>AEYCKMKKDYRKKYRKYVRSRFQCIEDRNARLGESVSLNKRYTRLRLIKEHRSQQEREQELLAIGKTKTCESPVSPIKMELLFDPDDEHSEPVHTVVFQGAAGIGKTILARKMMLDWASGTLYQDRFDYLFYIHCREVSLVTQRSLGDLIMSCCPDPNPPIHKIVRKPSRILFLMDGFDELQGAFDEHIGPLCTDWQKAERGDILLSSLIRKKLLPEASLLITTRPVALEKLQHLLDHPRHVEILGFSEAKRKEYFFKYFSDEAQARAAFSLIQENEVLFTMCFIPLVCWIVCTGLKQQMESGKSLAQTSKTTTAVYVFFLSSLLQPRGGSQEHGLCAHLWGLCSLAADGIWNQKILFEESDLRNHGLQKADVSAFLRMNLFQKEVDCEKFYSFIHMTFQEFFAAMYYLLEEEKEGRTNVPGSRLKLPSRDVTVLLENYGKFEKGYLIFVVRFLFGLVNQERTSYLEKKLSCKISQQIRLELLKWIEVKAKAKKLQIQPSQLELFYCLYEMQEEDFVQRAMDYFPKIEINLSTRMDHMVSSFCIENCHRVESLSLGFLHNMPKEEEEEEKEGRHLDMVQCVLPSSSHAACSHGLVNSHLTSSFCRGLFSVLSTSQSLTELDLSDNSLGDPGMRVLCETLQHPGCNIRRLWLGRCGLSHECCFDISLVLSSNQKLVELDLSDNALGDFGIRLLCVGLKHLLCNLKKLWLVSCCLTSACCQDLASVLSTSHSLTRLYVGENALGDSGVAILCEKAKNPQCN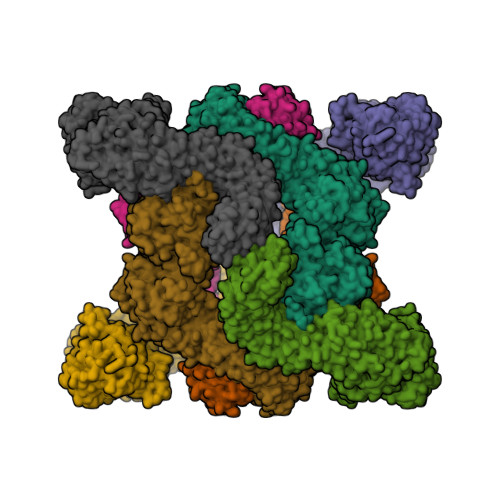LQKLGLVNSGLTSVCCSALSSVLSTNQNLTHLYLRGNTLGDKGIKLLCEGLLHPDCKLQVLELDNCNLTSHCCWDLSTLLTSSQSLRKLSLGNNDLGDLGVMMFCEVLKQQSCLLQNLGLSEMYFNYETKSALETLQEEKPELTVVFEPSW[8x]> GIILQTYRAIADYEKTSGSEMALSTGDVVEVVEKSESGWWFCQMKGKRGWIPASFLEP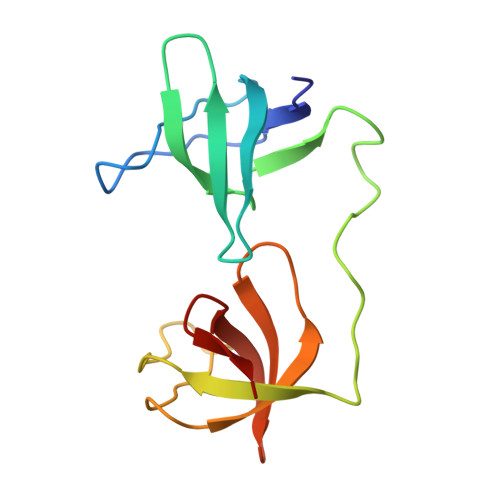LDSPDETEDPEPNYAGEPYVAIKAYTAVEGDEVSLLEGEAVEVIHKLLDGWWVIRKDDVTGYFPSMYLQKSGQ>ASNRKFFVGGNWKMNGSKESNQKLLKTLSDAKPDANTEILVAVPFVYLKDVREHLDKRFHVAAQNCYKVASGAFTGEISPAMIRDCGCEWVILGHSERRHIFGESDELIGEKVNHALTCGLKVVPCIGEKLDEREAGKTEQVCFRQLDAIKKGIPKAEDWSRVVIAYEPVWAIGTGKT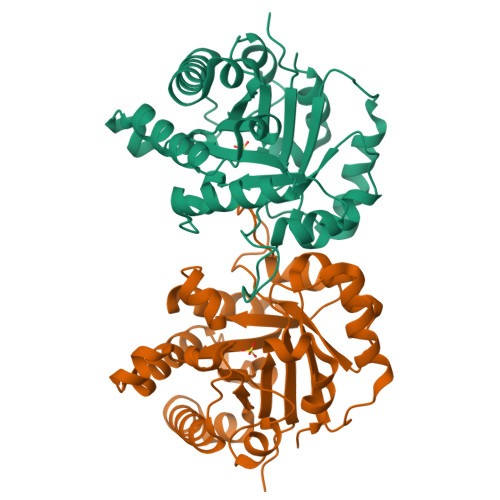ASPEQAQEVHHAVRQWLEKNVSQAVASSLRITYGGSVTAANCKELAKKPDVDGFLVGGASLKPEFVDICNAN[6x]> MNILKHFPSYVGPSKIRTLVIPIGHWT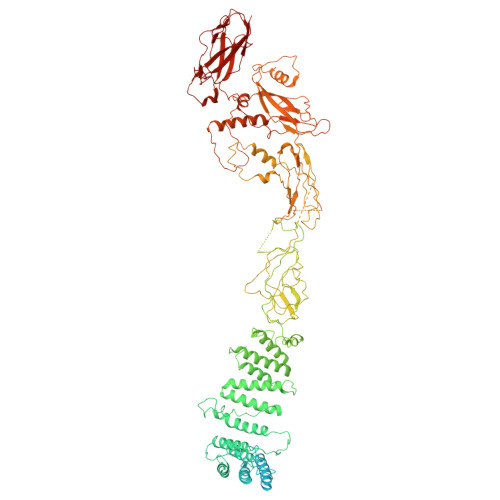RKEFNNAVQKLSEFNEIHLSDVTPIDSPIFTPQGFPHGKLFFDFLTIDHDDALELFLYDFEPFRKTFVIIGLVNDYSDPLTNLNFMKEKYPTLISPNLVYASSTPTKELEQTIDTMENVFASSPDMQKNIETIMCDIARNFLTALNSYYSSYKHVTLRSPGAIGGNAVLKTTLIRQNSYTSSSSSTPMSAVQSSVSSSSKAGSVTTASKRLSSFEMTTNSLKRSASLKLATTLSTSENRSQQKSLGRQMKILGNFQLLAGRYVDALNSFVDAITTLYKVRDYLWLGSALDGISICFLLLSYLGLSYQIPQIVSLICPVEKLNFESSSTGISPVDSNSKATASTTASSTPRNSISIAAMQSPRNSIMSLSAPALNIDVENINLPLLIKCISDKVLYYYDLSLMHNSEYAPQVVYCEFLLKTLTFMTSCYKSSEFSKDVLDNIVKNQHRALSDIPNSPMFPRFEVYFYSNKLFELQLKEMQVEAQIKIYSTMAEVYRLLGYKRKQLFVLRLLMVALLATPNKIAWHPDYRTLIDTIIELLNINESEAKINVDDPSQSTWLILQKKILQLCIKVSRKINDFEYVAKFSSILITKYTHLLNQSEQDALFKEYIQPSITNESITSYWDPFILREVVINRILDSDPTSNEIPLESDVSSLESLENRQKTQDINPQEVFNPFKRVQPTSFVSNNSTKVPILVFLVGDKAEFTCRVQNPFKFDFTINDIQLDEEISEFCEIDRKAVSYSGPYNVKAESIRSITLPLIIKKPTYKKIYEISCLKISILKLPLQKFDIINDSRRSNPVEEEAEYSKCIYGKLKIKILPEQPQLELLSTSKMTRNSWMMLDGTKTDFHITVRNKSLSCAINHIKIIPMNNIEQMLKPDYWKKMPPDDLYIMEKQLDWLSKSCVRIIKLPTVIKPNETITFDLELDNTAVPFNFTGFDLLIEYGMSATDESCIYLKKLSIPYEVTLRRTIEVPSMDIIPLNELFSSQVENVDWIEYVMSKIRAESNLHSRDFILLLLDFRNSWIDGIKLNVQFEDFTSNEYHVEASHTSRIIVPIKKIDYKKYNFENTPIPRIYPGRQFIQSGLNEEQTIEMRQKFWCREHIISKLKCNWKLTTDQSVTGSVDFNKFIEKFDHKMVYTIYPGRLFYGVQLLLDEPKVKVGEIINLKIITEPTSTCRRKQNSTVNFLDIVIFDSKTSKILPRSNRRILYNGSLTKPISTTKVSEINLEIIPIEKGRYEFSVCISKSNNQDGIIQFDSENVILSVI>MQNERSEQSMPGMPAPGLPAGFERRFSRRYAQLDDVRLHYVTGGPDDGEMVVLLHGWPQTWYTWRHVMPALAEDGYRVVAVDYRGAGESDKPLGGYDKASMAGDIRALVHQLGATRIHLVGRDIGVMVAYAYAAQWPTEIVKLAMLDVPVPGTRIWDEAKASADPQIWHFGLHQQRDIAEMLIAGKERAYILDFYKKRTHVALSNDDIAVYADAYAAPGALRAGFELYRAFPQDETRFKAFMKHKLPMPVLALAGDKSNGAKELDMARELALDVRGAVAPNTGHWLPDENPAFLTRQLLDFFREAASGR[4x]

Here we report the biochemical and structural characteristics of Cfl1 and Cfl2, two Cif-like epoxide hydrolases from Burkholderia cenocepacia. EHs that belong to the α/β hydrolase superfamily of enzymes utilize an Asp-His-Asp/Glu catalytic triad to open the epoxide ring substrate and release the vicinal diol product. Cfl1 and Cfl2 also appear to utilize a Cif-like His-Tyr epoxide ring-opening pair instead of the classical Tyr-Tyr pair. While Cif and aCif exist as constitutive dimers, our hydrodynamic and structural studies revealed that Cfl1 and Cfl2 exist as octamers and decamers, respectively, by forming rings of dimers.

Cfl1 is able to hydrolyze xenobiotic as well as biological epoxides that might be encountered in the environment or during infection. When we compared the Cfl1 and Cif active sites, we observed two unique features in Cfl1 (inset). First, Asp147, the Cfl1 residue presumed to be the charge-relay acid according to the pairwise sequence alignment with Cif, is not hydrogen bonded with His284, as is typical in acid-base-nucleophile catalytic triads. Instead, that hydrogen bond with His284 is satisfied by Ser258. The side chain of Asp147 is oriented in the opposite direction compared to Cif's Glu153 and forms a salt bridge with Arg122, which aligns to His128 in Cif. The second unique feature of the Cfl1 active site is that Arg122 forms a hydrogen bond with the catalytic water. The N-terminus of Cfl1 monomer 3 makes several electrostatic interactions with monomer 1, as well as a hydrophobic interaction mediated by the insertion of Met13 into a pocket comprised of Phe22, Phe26, Val41, Trp61, and the hydrocarbon portions of Glu23 and Arg28 side chains (cluster 1). The absence of this region in Cfl1 is a major reason that its dimer interface surface area is smaller compared to those of Cfl2, Cif, and aCif. Comparative NMA between the dimers of Cfl1, Cfl2, Cif, aCif showed that the ex circulum (i.e., out of the ring) dimer of Cfl1 with its smallest dimer interface is the most flexible. We hypothesize that Cfl1, but not Cfl2, retains sufficient intra-monomer flexibility in circulum to achieve substantial catalytic activity.>ADQSFLWNVFQRVDKDRSGVISDTELQQALSNGTWTPFNPVTVRSIISMFDRENKAGVNFSEFTGVWKYITDWQNVFRTYDRDNSGMIDKNELKQALSGYRLSDQFHDILIRKFDRQGRGQIAFDDFIQGCIVLQRLTD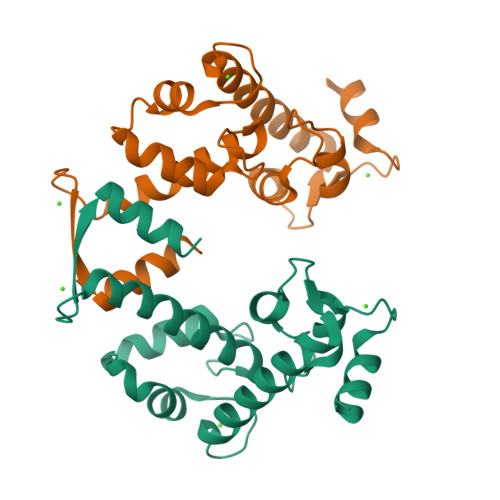IFRRYDTDQDGWIQVSYEQYLSMVFSIV[2x]> GVATHGGSYVQYNVYGNLFEVSRKYVPPLRPIGRGAYGIVCAATNSETGEEVAIKKIGNAFDNIIDAKRTLREIKLLKHMDHENVIAVKDIIKPPQRENFNDVYIVYELMDTDLHQIIRSNQPLTDDHCRFFLYQLLRGLKYVHSANVLHRDLKPSNLLLNANCDLKLGDFGLARTKSETDFMTEYVVTRWYRAPELLLNCSEYTAAIDIWSVGCILGETMTREPLFPGKDYVHQLRLITELIGSPDDSSLGFLRSDNARRYVRQLPQYPRQNFAARFPNMSAGAVDLLEKMLVFDPSRRITVDEALCHPYLAPLHDINEEPVCVRP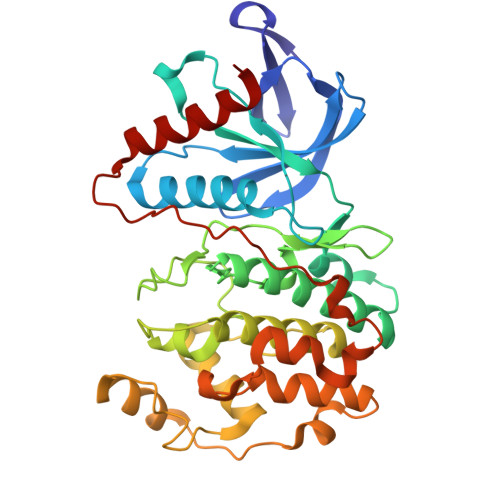FNFDFEQPTLTEENIKELIYRETVKFNP>MVHATSPLLLLLLLSLALVAPGLSARKCSLTGKWTNDLGSNMTIGAVNSRGEFTGTYITAVTATSNEIKESPLHGTQNTINKRTQPTFGFTVNWKFSESTTVFTGQCFIDRNGKEVLKTMWLLRSSVNDIGDDWKATR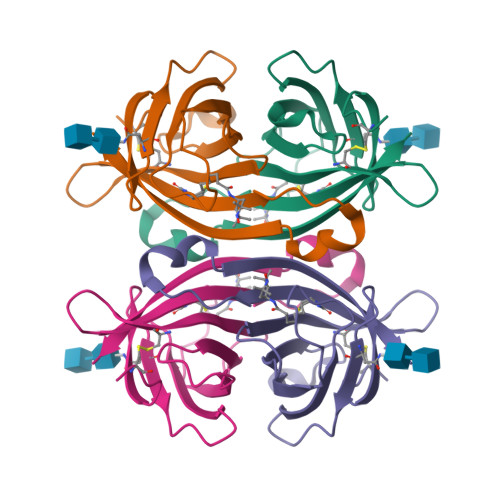VGINIFTRLRTQKE[4x]>VKLAGNSSLCPVSGWAIYSKDNSVRIGSKGDVFVIREPFISCSPLECRTFFLTQGALLNDKHSNGTIKDRSPYRTLMSCPIGEVPSPYNSRFESVAWSASACHDGINWLTIGISGPDSGAVAVLKYNGIITDTIKSWRNNILRTQESECACVNGSCFTIMTDGPSDGQASYKIFRIEKGKIVKSVEMNAPNYHYEECSCYPDSSEITCVCRDNWHGSNRPWVSFNQNLEYQIGYICSGVFGDNPRPNDKTGSCGPVSSNGANGVKGFSFKYGNG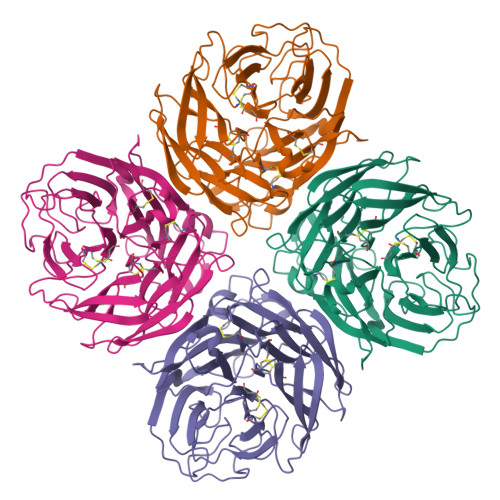VWIGRTKSISSRKGFEMIWDPNGWTGTDNNFSIKQDIVGINEWSGYSGSFVQHPELTGLDCIRPCFWVELIRGRPEENTIWTSGSSISFCGVNSDTVGWSWPDGAELPFTI[4x]>[2x]GSSHHHHHHSSGLVPRGSMSTSWSDRLQNAADMPANMDKHALKKYRREAYHRVFVNQSLAMEKIKCFGFNMDYTLAVYKSPEYESLGFELTVERLVSIGYPQELLSFAYDSTFPTRGLVFDTLYGNLLKVDAYGNLLVCAHGFNFIRGPETREQYPNKFIQRDDTERFYILNTLFNLPETYLLACLVDFFTNCPRYTSCETGFKDGDLFMSYRSMFQDVRDAVDWVHYKGSLKEKTVENLEKYVVKDGKLPLLLSRMKEVGKVFLATNSDYKYTDKIMTYLFDFPHGPKPGSSHRPWQSYFDLILVDARKPLFFGEGTVLRQVDTKTGKLKIGTY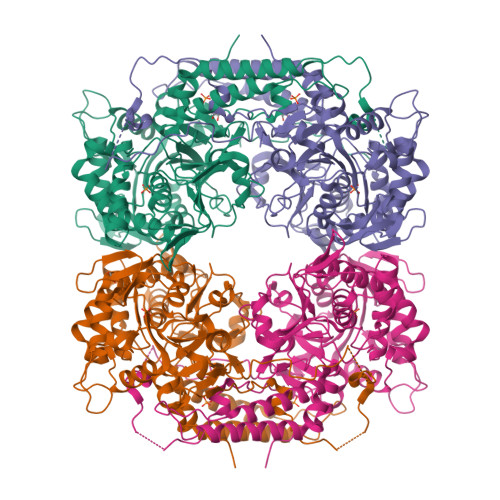TGPLQHGIVYSGGSSDTICDLLGAKGKDILYIGDHIFGDILKSKKRQGWRTFLVIPELAQELHVWTDKSSLFEELQSLDIFLAELYKHLDSSSNERPDISSIQRRIKKVTHDMDMCYGMMGSLFRSGSRQTLFASQVMRYADLYAASFINLLYYPFSYLFRAAHVLMPHESTVEHTHVDINEMESPLATRNRTSVDFKDTDYKRHQLTRSISEIKPPNLFPLAPQEITHCHDEDDDEEEEEEEE> SSEKEY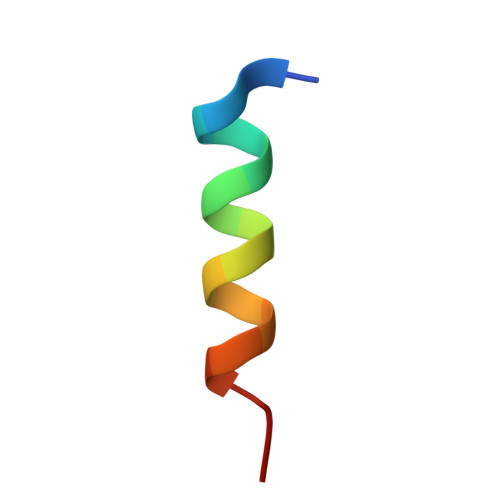VEMLDRLYSKLP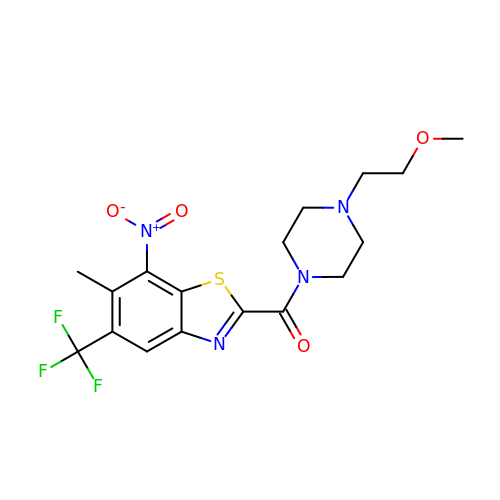[4-(2-methoxyethyl)piperazin-1-yl][6-methyl-7-nitro-5-(trifluoromethyl)-1,3-benzothiazol-2-yl]methanone | C17 H19 F3 N4 O4 S | AOMUWGOWJLARPE-UHFFFAOYSA-N> VMPIVRVAVLAAGDDGGRLTEMALPSELPLREILPAVQRIVQPARENDGAADPAAAPNPVRLSLAPIGGAPFSLDATLDTVGVVDGDLLALQAVPSGPPAPRIVEDIADAAVIFSEARRRQWGPTHIARGAALALIGLILVGTGLSVAHRVITGDLLGQFIVSGIALATVIAALAVRNRSAVLATSLAVTALVPVAAAFALGVPGDFGAPNVLLAAAGVAAWSLISMAGSPDDRGIAVFTATAVTGVGVLLVAGAASLWVISSDVI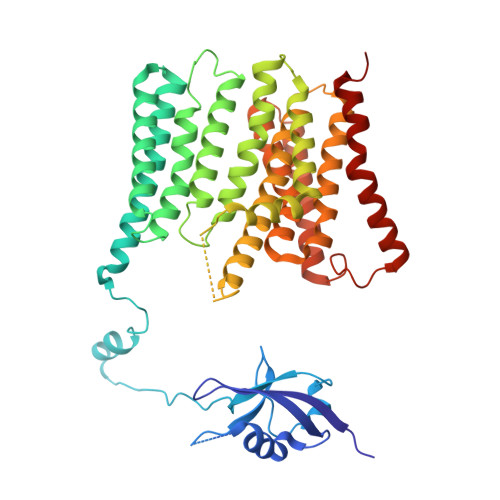GCALVLLGLIVTVQAAQLSAMWARFPLPVIPAPGDPTPAARPLSVLADLPRRVRVSQAHQTGVIAAGVLLGVAGSVALVSSANASPWAWYIVVAAAAGAALRARVWDSAACKAWLLGHSYLLAVALLVAFVIGDRYQAALWALAALAVLVLVWIVAALNPKIASPDTYSLPMRRMVGFLATGLDASLIPVMALLVGLFSLV>ASPTSPKVFPLSLCSTQPDGNVVIACLVQGFFPQEPLSVTWSESGQGVTARNFPPSQDASGDLYTTSSQLTLPATQCLAGKSVTCHVKHYTNPSQDVTVPCPVPSTPPTPSPSTPPTPSPSCCHPRLSLHRPALEDLLLGSEANLTCTLTGLRDASGVTFTWTPSSGKSAVQGPPERDLCGCYSVSSVLPGCAEPWNHGKTFTCTAAYPESKTPLTATLSKSGNTFRPEVHLLPPPSEELALNELVTLTCLARGFSPKDVLVRWLQGSQELPREKYLTWASRQEPSQGTTTFAVTSILRVAAEDWKKGDTFSCMVGHEALPLAFTQKTIDRLAGKPTHVNVSVVMAEVDGTCY[4x];> KSPIFGPEEVNSVEGNSVSITCYYPPTSVNRHTRKYWCRQGARGGCITLISSEGYVSSKYAGRANLTNFPENGTFVVNIAQLSQDDSGRYKCGLGINSRGLSFDVSLEVSQGPGLLNDTKVYTVDLGRTVTINCPFKTENAQKRKSLYKQIGLYPVLVIDSSGYVNPNYTGRIRLDIQGTGQLLFSVVINQLRLSDAGQYLCQAGDDSNSNKKNADLQVLKPEPELVYEDLRGSVTFHCALGPEVANVAKFLCRQSSGENCDVVVNTLGKRAPAFEGRILLNPQDKDGSFSVVITGLRKEDAGRYLCGAHSDGQLQEGSPIQAWQLFVNEESTIPRSPTVVKGVAGGSVAVLCPYNRKESKSIKYWCLWEGAQNGRCPLLVDSEGWVKAQYEGRLSLLEEPGNGTFTVILNQLTSRDAGFYWCLTNGDTLWRTTVEIKIIEGEPNLKVPGNVTAVLGETLKVPCHFPCKFSSYEKYWCKWNNTGCQALPSQDEGPSKAFVNCDENSRLVSLTLNLVTRADEGWYWCGVKQGHFYGETAAVYVAVEERHHHHHH;> QEDERIVLVDNKCKCARITSRIIRSSEDPNEDIVERNIRIIVPLNNRENISDPTSPLRTRFVYHLSDLCKKCDPTEVELDNQIVTATQSNICDEDSATETCYTYDRNKCYTAVVPLVYGGETKMVETALTPDACYPD;>[2x]QEGDFPMPFISAKSSPVIPLDGSVKIQCQAIREAYLTQLMIIKNSTYREIGRRLKFWNETDPEFVIDHMDANKAGRYQCQYRIGHYRFRYSDTLELVVTGLYGKPFLSADRGLVLMPGENISLTCSSAHIPFDRFSLAKEGELSLPQHQSGEHPANFSLGPVDLNVSGIYRCYGWYNRSPYLWSFPSNALELVVTAIDGRAHHHHHH

Immunoglobulin (Ig) A functions as monomeric IgA in the serum and Secretory (S) IgA in mucosal secretions. Host IgA Fc receptors (FcαRs), including human FcαR1/CD89, mediate IgA effector functions; however, human pathogen Streptococcus pyogenes has evolved surface-protein virulence factors, including M4, that also engage the CD89-binding site on IgA. SIgA is polymeric and is typically composed of two mIgA that assemble with one joining-chain (JC) to form dimeric (d) IgA, which is bound by the polymeric Ig-receptor (pIgR) ectodomain, called secretory component (SC). Here we report cryo-EM structures of M4-SIgA and CD89-SIgA complexes, which unexpectedly reveal different SIgA-binding stoichiometry for M4 and CD89.

The ectodomain of CD89 consists of two immunoglobulin-like domains (D1 and D2) arranged at an angle of approximately 90° to each other. Map quality and resolution were sufficient to refine the positions of main chain and side chain atoms for the residues at the interface, while density in the distal region of CD89, including the second Ig-like domain D2, was of lower resolution. The refined structure revealed a 2:1 CD89:SIgA binding stoichiometry verifying that two copies of CD89 can bind both mIgA and SIgA. The two copies of CD89 bound to SIgA are separated by 108 Å (distance between the two copies of D2 C-terminal residue T195) and relative to each other are oriented differently than the two CD89 bound to mIgA for which C-terminal residues are reportedly spaced by 124 Å. Alignment to the mIgA-CD89 structure revealed superimposable binding sites (RMSD = 1.165 at FcAB; RMSD = 1.121 at FcCD) on Cα2 and Cα32. Consistent with the mIgA-CD89 structure, the CD89 D1 BC loop, the D strand, the DE loop, and the FG loop (Ig-like domain nomenclature) contacted a total of 19 IgA residues, including three Cα2 residues and 16 Cα3 residues, burying a total of 1656 Å2. A comparison of the CD89 and M4 binding footprints on SIgA revealed five shared interface residues (E389, L441, F443, T444, Q445) located on the Cα3 domain. CD89 binds additional residues located toward and on Cα2, whereas M4 contacts only Cα3 and binds residues closer to the Tps and JC, including R346, T447, D449 from HC-A and S356, E357, A360 from HC-B. CD89 and M4’s distinct binding footprints and structures direct CD89 D2 C-terminal residues away from SIgA and direct the M4 fragment C-terminal residues (and likely the rest of the M4 coiled-coil), alongside FcAB in a line near parallel to Cα3.> GAMAPPFFDLKPVSVDLALGESGTFKCHVTGTAPIKITWAKDNREIRPGGNYKMTLVENTATLTVLKVTKGDAGQYTCYASNVAGKDSCSAQLGVQEPPRFIKKLEPSRIV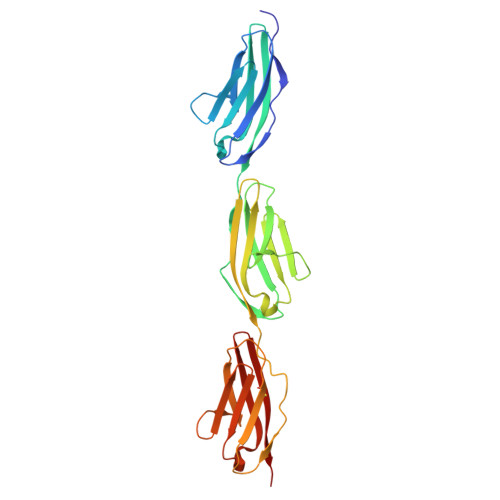KQDEHTRYECKIGGSPEIKVLWYKDETEIQESSKFRMSFVESVAVLEMYNLSVEDSGDYTCEAHNAAGSASSSTSLKVKEPPVFRKKPHPVETLKGADVHLECELQGTPPFQVSWHKDKRELRSGKKYKIMSENFLTSIHILNVDSADIGEYQCKASNDVGSYTCVGSITLKA>GMSDLKSLATKFASDHESGKLLVLPTVWDTWSAGL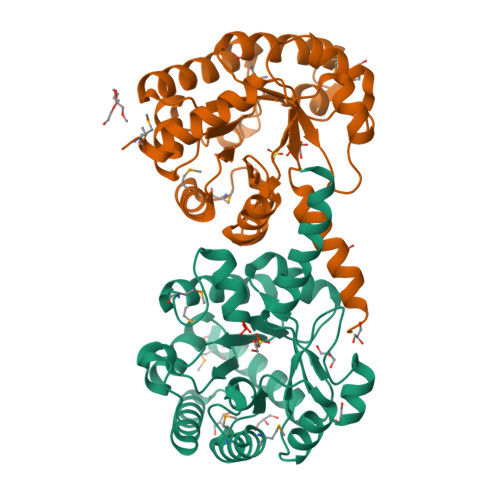VEEAGFSGLTIGSHPVADATGSSDGENMNFADYMAVVKKITSAVSIPVSVDVESGYGLSPADLIAQILEAGAVGINVEDVVHSEGKRVREAQEHADYIAAARQAADVAGVDVVINGRTDAVKLGADVFEDPMVEAIKRIKLMEQAGARSVYPVGLSTAEQVERLVDAVSVPVNITAHPVDGHGAGDLATLAGLGVRRVTFGPLWQKWLAATSAQQLKGWA[2x]N~2~-(biphenyl-4-ylsulfonyl)-N-hydroxy-N~2~-(2-hydroxyethyl)glycinamide | C16 H18 N2 O5 S | 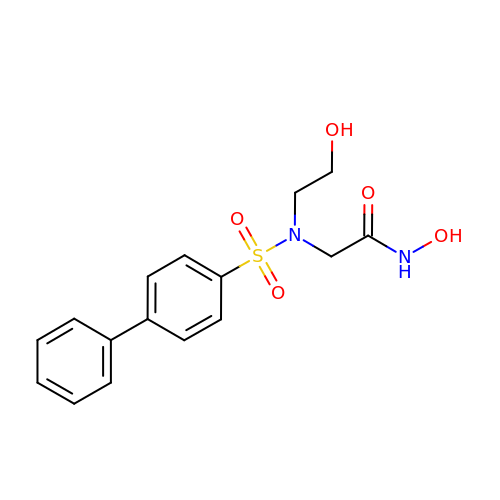QQDWEVONJRXVDB-UHFFFAOYSA-N>[2x]MASKKVCIVGSGNWGSAIAKIVGGNAAQLAQF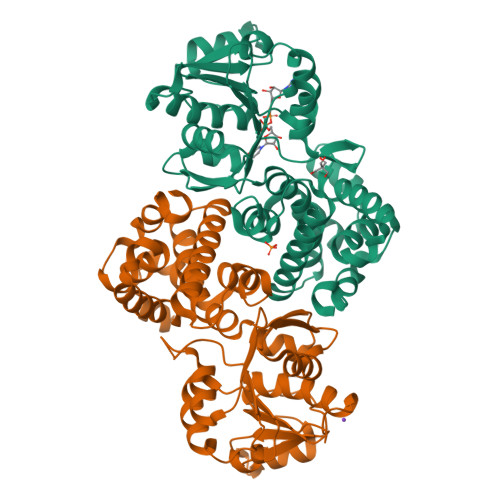DPRVTMWVFEEDIGGKKLTEIINTQHENVKYLPGHKLPPNVVAVPDVVQAAEDADILIFVVPHQFIGKICDQLKGHLKANATGISLIKGVDEGPNGLKLISEVIGERLGIPMSVLMGANIASEVADEKFCETTIGCKDPAQGQLLKELMQTPNFRITVVQEVDTVEICGALKNVVAVGAGFCDGLGFGDNTKAAVIRLGLMEMIAFAKLFCSGPVSSATFLESCGVADLITTCYGGANRKVAEAFARTGKSIEQLEKELLNGQKLQGPETARELYSILQHKGLVDKFPLFMAVYKVCYEGQPVGEFIHCLQNHPEHM1-(1-{(2S)-3-[(6-chloronaphthalen-2-yl)sulfonyl]-2-hydroxypropanoyl}piperidin-4-yl)tetrahydropyrimidin-2(1H)-one 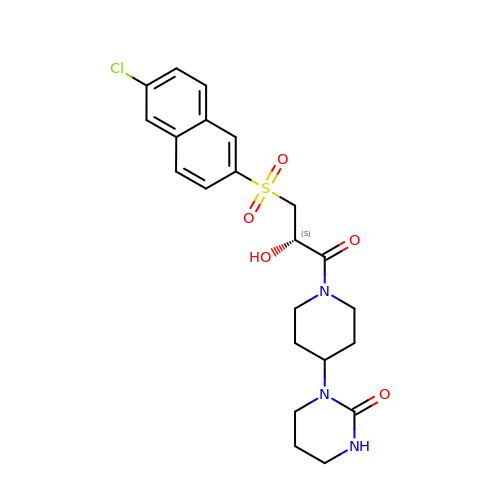| C22 H26 Cl N3 O5 S | GEHAEMCVKDPMKO-HXUWFJFHSA-N>MGHHHHHHKKIDDDLFEELEEQLLIADVGVETTRKIITNLTEGASRKQLRDAEALYGLLKEEMGEILAKVDEPLNVEG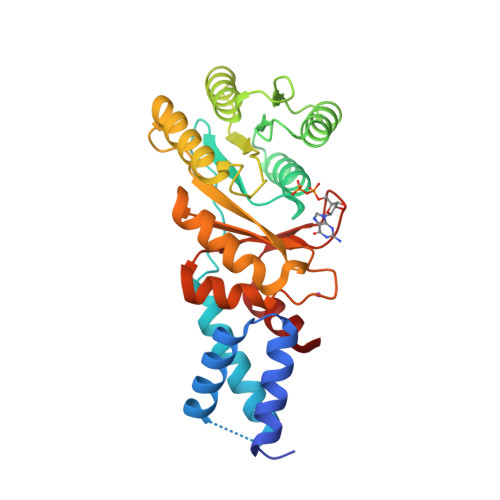KAPFVILMVGVNGVGKTTTIGKLARQFEQQGKSVMLAAGDTFRAAAVEQLQVWGQRNNIPVIAQHTGADSASVIFDAIQAAKARNIDVLIADTAGRLQNKSHLMEELKKIVRVMKKLDVEAPHEVMLTIDASTGQNAVSQAKLFHEAVGLTGITLTKLDGTAKGGVIFSVADQFGIPIRYIGVGERIEDLRPFKADDFIEALFARED[2x]> MGCPFSQSVSQPVDERLTRAAIFLVVTINPGKAAEVAVRAHCSILSSLIRGVGFRISDGGLSCVMGVSEGGWERLFGDTKPEYLHVFREINGVHHAPSTPGDLLYHIRAARMDLCFELASRILSDLGNSVSVVDSVQGFRYFDDRDLLGFVDGTENPVAQAA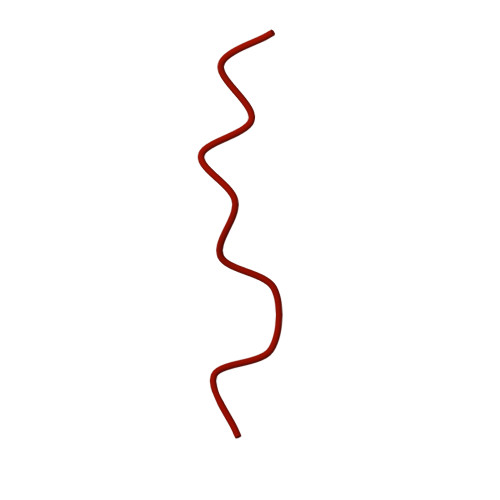VDATLIGDEDMVFAGGSYVIVQKYLHDLDKWNAIPVEQQEKIIGREKLSDIELRDADKPSYAHNVLTSIEEDGEDVDILRDNMPFGDPGKGEFGTYFIGYSRKPERIERMLENMFIGNPPGNYDRILDVSRAITGTLFFVPTTSFLDSIEPQSAPGQQGDDVINTLRSTAIKGDIMPGSLNIGSLKKEV> AESTTLETI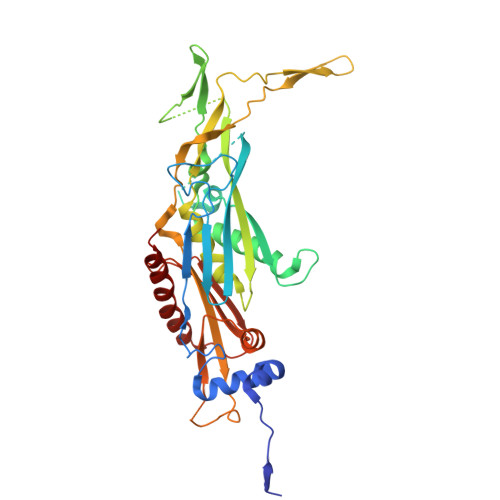EIHPITFPPEVLARISPELSLQRHLSLGIRPCLRKYEEFRDVAIENNTLSRYADAGNIDTKNNILGSNVLKSGKTIVITSITGGIIEETSASIKDLDDFGEEELFEVTKEEDIIANYASVYPVVEVERGRVGACTDEEMTISQKLHDSILHSRILPKKALKVKAGVRSANEDGTFSVLYPDELEDDTLNETNLKMKRKWSYVLYAKIVVLSRTGPVFDLCWNSLMYALQSVKLPRAFIDERASDLRMTIRTRGRSATIRETYEIICDQTKSVPLMINAKNIAFASNYGIVELDPECQLQNSDNSEEEEVDIDMDKLNTVLIADLDTEAEETSIHSTISILAAPSGNYKQLTLMGGGAKITPEMIKRSLLLSRVRADDLSTRFNI One such assembly is the Ctf19c/CCAN, which anchors the kinetochore on chromosomal DNA. There are 13 Ctf19c subunits (Pekgöz Altunkaya et al., 2016), and these associate with a second complex containing Mif2/CENP-C and the Cse4/CENP-A nucleosome. We present here the structure of the Ctf19c determined by cryo-EM. The structure provides an overview of the inner kinetochore and the coordination of its various functions by showing how Ctf19c components are organized relative to each other, how this organization positions defined Cse4/CENP-A recognition elements, and how the Ctf19c supports regulated recruitment of outer kinetochore proteins that tether the chromosome to the microtubule tip.

We assembled the Ctf19c from individual parts (Ame1-Okp1, Ctf19-Mcm21, Nkp1-Nkp2, Chl4-Iml3, Ctf3-Mcm16-Mcm22, and Cnn1-Wip1) and purified the recombinant complex to homogeneity by size exclusion chromatography. We used these images to determine the structure of the Ctf19c to an overall resolution of ~4.2 Å. A twofold symmetry axis in the calculated density map related equivalent sides, which were separated by a central cavity. A refined map corresponding to a single Ctf19c protomer showed amino acid side chain density for much of the complex, guiding modeling of individual polypeptide chains and their interactions. For the Ctf3c and for parts of COMA that are not well-resolved, we fit the density with poly-alanine chains and numbered the residues according to their approximate positions. The structure shows that, rather than a network of binary interactions, the Ctf19c/CCAN is a defined complex in which subunits interdigitate. C-terminal parts of Okp1 Ame1, Nkp1 and Nkp2 form a parallel, four-chain, helical coil. Our density map showed that yeast Chl4 shares these structural features and also enabled modeling of the Chl4 linker domain, which connects the two previously-described functional modules and provides extensive contacts between Chl4 and Ctf19-Mcm21. The map also showed density corresponding to the β3-β4 loop, which extends into the Ctf19c central cavity and contacts the Ame1-Okp1 coiled-coil. The Ctf3 trimer (Ctf3, Mcm16, and Mcm22) and the Cnn1-Wip1 dimer form a complex that recruits the microtubule-binding Ndc80 complex to the kinetochore through a flexible N-terminal extension of Cnn1. In addition to contact with Mcm21-Ctf19, which is described above, Ctf3 contacts Iml3 through a network of bulky residues in both proteins that fixes the position of the Ctf3c relative to Iml3.

> SNAMPYTWKFLGISKQLSLENGIAKLNQLLNLEVDLDIQTIRVPSDPDGGTAADEYIRYEMRLDISNLDEGTYSKFIFLGNSKMEVPMFLCYCGTDNRNEVVLQWLKAEYGVIMWPIKFEQKTMIKLADASIVHVTKENIEQITWFSSKLYFEPETQDKNLRQFSIEIPRESCEGLALGYGNTMHPYNDAIVPYIYNETGMAVERLPLTSVILAGHTKIMRESIVTSTRSLRNRVLAVVLQSIQFTSE;> SNAMSRIDDLQQDIESLLSEINSLEESREKLKAKIKDKRKNEESANPIVQEFEDLFDQFPQLNNFLFNEHPELEETDDKDISRAQADIPATPIPYEPKKRAKLENEEILPEQEWVLKTQPMVQHQMFDPGVADLLDTDILTSPSKRKRKLKIDDISTSDRSELEDYIVLENVYRMFGITFFPLVDPIDLKIKDASGEIFVDREMLGIRLEVFSERTSQFEKPHYVLLKKRIKSNSWFLFKHTIPSFIDVQGIFDDTNGGLVISHDDAYLFAKRVFLQLVEVQKRRQIFKDLEAKKIIHDLDLDLESSMVSFFVKDIKVELFVKQNEIVSCSILDDIHDFSQNNKSKWEIALLGSLDDLELKLNHSFATIFK;> MDFTSDTTNSHDTSNSHLSLEDAVGTHHAGEADVNIDGDEKQQLSLLDDDQVRALKLQEEKDALLTRRNTLLQEIQTYQNILMKENNSKTKNGDILQNDITQDFLNLISISSSNPNSAISDRKRVERINGLTNLQKELVTKYDTLPLLNMNLRLSYLRDHTYPHLQVSVQSRDRVHNDGIEVLVVNYKFCRNTMNPFEIQFKMFYKFEDSTLLKWEILRISTNVRLKAKQLLATRNFQKCLLSLYEFDKIKSKKTGIFQNLINLLKRKTRCYLMNNSDSLIVERVIREGRLTTIKLQINFIITMPGERGKPRNCFLPMSKISIALWKGGERFNQIDLDEICYGLIKEYGVKTGLKEICNVCLFPDMYAR;> SNAMSNELRLEDNYVPTSDTLVVFKQLMKLPVTVLYDLTLSWFAKFGGSFDGDIYLLTETLDLLIEKGVRRNVIVNRILYVYWPDGLNVFQLAEIDCHLMISKPEKFKWLPSKALRGDGKPYVVKLQPAKFIENLQTDLAKIYHCHVYMFKHPSLPVLITRIQLFDSNNLFLSTPNIGSINKESLYNKLDKFQGKPLISRRPYYVAFPLNSPIIFHSVDKDIYARLVLQSISRTISERETIIFKPVQKIPVKSIHNIMTLLGPSRFAESMGPWECYASANFERSPLHDYKKHQGLTGKKVMVREFDDSFLNDDENFYGKEEPEIRRLRLEKNMIKFKGSANGVMDQKYNDLKEFNEHVHNIRNGKKNEDSGEPVYISRYSSLVPIEKVGFTLKNEINSRIITIKLKFNGNDIFGGLHELCDKNLINIDKVPGWLAGENGSFSGTIMNGDFQREQVAKGGLL;> MAADRDNFLQNIENDSINNGQAMDLSPNRSSSESDSSILMNVNDIKTLRLDVAPEAKSTQSKKSLFYENSDDAEEGEIEERTNKEEGQYHHKGSKQLRFEVGKESTGKLQSHLSDGSATSGEGNVRPWEFRKVIQAEYRERLPRNYELKHWKKPSKIMIGSILRLLETNTVSALDSVFEKYEKEMNQMTHGDNNEVKRIYSKKERLLEIILTKIKKKLRQAKFPSRISERDLDIEYIYSKRQFIQNRYSQELQNNERLEAILSREQNLLEETRKLCMNLKTNNKKRLTEKLIQKDLHPVLNKAMEYTYGLESTNGFMHPDGPVTFRNDSHELNLMLNDPIKSTADVRLDKEEVLSLLPSLKEYTKKSKELKETMGQMISDSHEEEIKEVFVPHHESHQDKTEEDIH;> SNAMTDTYNSISNFIENELTALLSSDDYLMDDLAGELPNEVCRLLKAQVIEKRKDAMSRGKQDLLSKEIYDNESELRASQSQQIMELVGDIPKYSLGSELRNRVEGEPQSTSIERLIEDVLKLPQMEVADEEEVEVENDLKVLSEYSNLRKDLILKCQALQIGESKLSDILSQTNSINSLTTSIKEASEDDDISEYFATYNGKLVVALEEMKLLLEEAVKTFGNSPEKREKIKKILSELKK;>SNAMSLILDDIILSLTNANERTPPQALKTTLSLLYEKSKQYGLSSPQLQALVRLLCETSIIDTVTKVYIVENCFLPDGYLTKELLLEIINHLGTPTVFSRYRIQTPPVLQSALCKWLVHVYFLFPVHSEREHNISSSIWLHLWQFSFLQKWITPLVIWQATTPVDVKPWKLSIIKRCAMHPGYRDAPGSATLILQRFQCLVGASSQITESIITINCNRKTLKSHRNLKLDAHFLSILKRILSRAHPANFPADTVQNTIDMYLSEIHQLGADSIYPLRLQSLPEYVPSDSTVSLWDVTSLEQLAQNWPQLHIPNDVDYMMKPSLNSNVLLPRKVMSRDSLKHLYSSIILIKNSRDESSSPYEWCIWQLKRCFAHQIETPQEVIPIIISVSSMDNKLSSRIIQTFCNLKYLKLDELTLKKVCGGILPLWKPELISGTREFFVKFMASIFMWSTRDGHDNNCTFSETCFYVLQMITNWVLDDKLIALGLTLLHDMQSLLTLDKIFNNATSNRFSTMAFISSLDILTQLSKQTKSDYAIQYLIVGPDIMNKVFSSDDPLLLSAACRYLVATKNKLMQYPSTNKFVRMQNQYIMDLTNYLYRNKVLSSKSLFGVSPDFFKQILENLYIPTADFKNAKFFTITGIPALSYICIIILRRLETAENTKIKFTSGIINEETFNNFFRVHHDEIGQHGWIKGVNNIHDLRVKILMHLSNTANPYRDIAAFLFTYLKSLSKYSVQNSXXXXXXXXXXXXXXXXXXXXXXXXXXXXXXXXXXXXX[2x];> MDRDTKLAFRLRGSHSRRTDDIDDDVIVFKTPNAVYREENSPIQSPVQPILSSPKLANSFEFPITTNNVNAQDRHEHGYQPLDAEDYPMIDSENKSLISESPQNVRNDEDLTTRYNFDDIPIRQLSSSITSVTTIDVLSSLFINLFENDLIPQALKDFNKSDDDQFRKLLYKLDLRLFQTISDQMTRDLKDILDINVSNNELCYQLKQVLARKEDLNQQIISVRNEIQELKAGKDWHDLQNEQAKLNDKVKLNKRLNDLTSTLLGKYEGDRKIMSQDSEDDSIRDDSNILDIAHFVDLMDPYNGLLKKINKINENLSNELQPSLHHHHHH;> MNSEQLLHNYVSDSLLTTLISFQEFKQQLQSYTSDEQQLQHWYELLQARDARVTSELEARIKQFFITLRSRLLRFLESEQLSHSLSLETLIDALYKINDLLQQRLQILDDAIQEKTSELAEFENMVRSPSAGDNAIPGLLQIIQSYINLLEEN>[4x]GSMPDYVAKYPVIQTDDE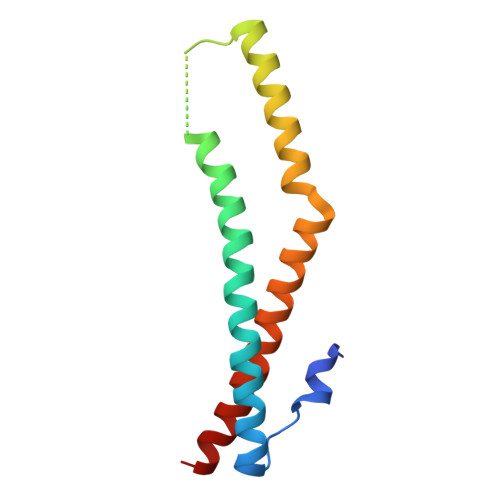RERYKAVFQDQFSEYKELSAEVQAVLRKFDELDAVMSRLPHHSESRQEHERISRIHEEFKKKKNDPTFLEKKERCDYLKNKLSHIKQRIQEYDKVMN> HHHHHHENLYFQGSGSSPRSGVLLRGCPTHCHCEPDGRMLLRVDCSDLGLSELPSNLSVFTSYLDLSMNNISQLLPNPLPSLRFLEELRLAGNALTYIPKGAFTGLYSLKVLMLQNNQLRHVPTEALQNLRSLQSLRLDANHISYVPPSCFSGLHSLRHLWLDDNALTEIPVQAFRSLSALQAMTLALNKIHHIPDYAFGNLSSLVVLHLHNNRIHSLGKKCFDGLHSLETLDLNYNNLDEFPTAIRTLSNLKELGFHSNNIRSIPEKAFVGNPSLITIHFYDNPIQFVGRSAFQHLPELRTLTLNGASQITEFPDLTGTANLESLTLTGAQISSLPQTVCNQLPNLQVLDLSYNLLEDLPSFSVCQKLQKIDLRHNEIYEIKVDTFQQLLSLRSLNLAWNKIAIIHPNAFSTLPSLIKLDLSSNLLSSFPITGLHGLTHLKLTGNHALQSLISSENFPELKVIEMPYAYQCCAFGVCENAYKISNQWNKGDNSSMDDLHKKDAGMFQAQDERDLEDFLLDFE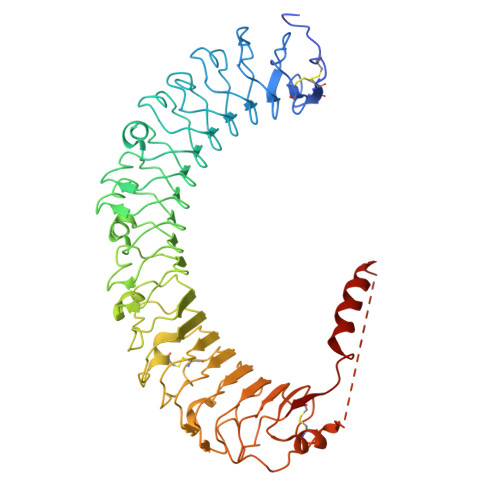EDLKALHSVQCSPAAA> SQIPASEQETLVR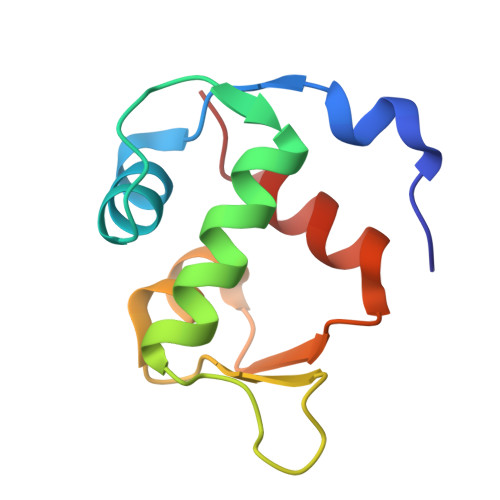PKPLLLKLLKSVGAQKDTYTMKEVLFYLGQYIMTKRLYDAAQQHIVYCSNDLLGDLFGVPSFSVKEHRKIYTMIYRNLV>GGAGCGGUAGUUCAGUCGGUUAGAAUACCUGCC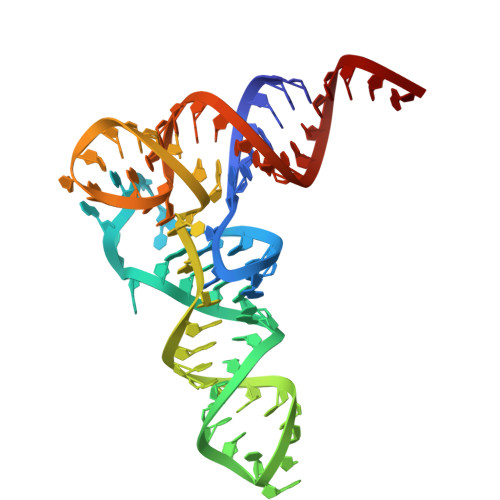UGUCACGCAGGGGGUCGCGGGUUCGAGUCCCGUCCGUUCCGCCA[2x]> ASLTEIEHLVQSVCKSYRETCQLRLEDLLRQRSNIFSREEVTGYQRKSMWEMWE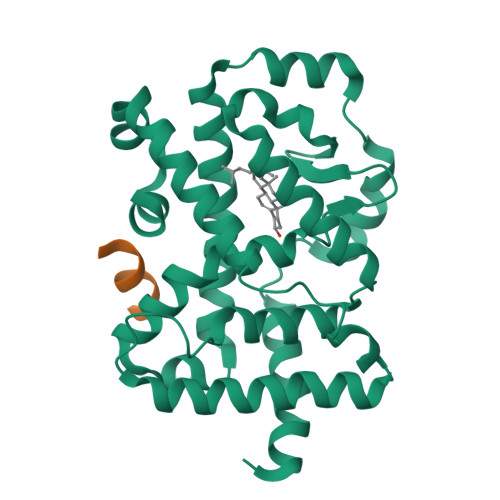RCAHHLTEAIQYVVEFAKRLSGFMELCQNDQIVLLKAGAMEVVLVRMCRAYNADNRTVFFEGKYGGMELFRALGCSELISSIFDFSHSLSALHFSEDEIALYTALVLINAHRPGLQEKRKVEQLQYNLELAFHHHLCKTHRQSILAKLPPKGKLRSLCSQHVERLQIFQHLHPIVVQAAFPPLYKELFS;> KILHRLLQDS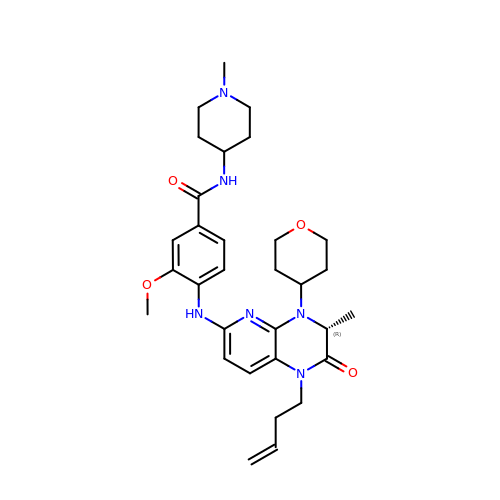4-{[(3R)-1-(but-3-en-1-yl)-3-methyl-4-(oxan-4-yl)-2-oxo-1,2,3,4-tetrahydropyrido[2,3-b]pyrazin-6-yl]amino}-3-methoxy-N-(1-methylpiperidin-4-yl)benzamide | C31 H42 N6 O4 | YEZKKIMJJAQTOO-OAQYLSRUSA-N>SEDCENIFHDNAYLLKLDCEAGRVDPVEYDDISDEEIYEITVDVGVSSEDQEKVAKIIRECIAQVSTQDCTKFSEIYDCYMKKKICNYYPENMGSGHHHHHHHH[2x];>KCPQPKTLDEFTIIQNLQPQYQFRDYFIATCKQGYQLIEGNQVLHSFTAVCQDDGTWHRAMPRCKIKDCGQPRNLPNGDFRYTTTMGVNTYKARIQYYCHEPYYKMQTRAGSRESEQGVYTCTAQGIWKNEQKGEKIPRCLPVCGKPVNPVEQRQRIIGGQKAKMG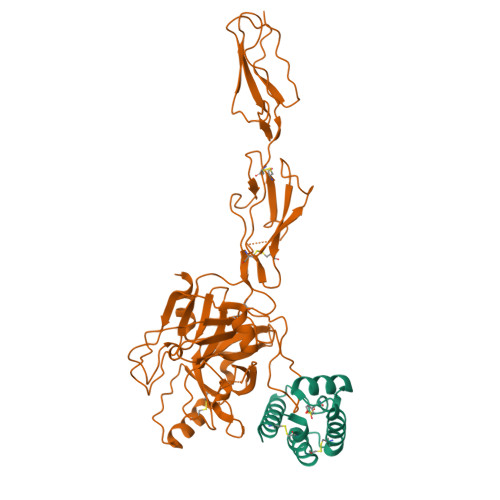NFPWQVFTNIHGRGGGALLGDRWILTAAHTLYPKEHEAQSNASLDVFLGHTNVEELMKLGNHPIRRVSVHPDYRQDESYNFEGDIALLELENSVTLGPNLLPICLPDNDTFYDLGLMGYVSGFGVMEEKIAHDLRFVRLPVANPQACENWLRGKNRMDVFSQNMFCAGHPSLKQDACQGDAGGVFAVRDPNTDRWVATGIVSWGIGCSRGYGFYTKVLNYVDWIKKEMEEEDGSGHHHHHHHH[2x]>[2x]MGADDVVDSSKSFVMENFSSYHGTKPGYVDSIQKGIQKPKSGTQGNYDDDWEGFYSTDNKYDAAGYSVDNENPLSGKAGGVVKVTYPGLTKVLALKVDNAETIKKELGLSLTEPLMEQVGTEEFIKRFGDGASRVVLSLPFAEGSSSVKYINNWEQAKALSVELEINFETRGKRGQDAMYEYMAQACAGNRVRRSVGSSLSCINLDWDVIRDKTKTKIESLKEQGPIKNKMSESPNKTVSEEKAKQYLEEFHQTALEQPELSELKTVTGTNPVFAGANYAAWAVNVAQVIDSETADNLEKTTAALSILPGIGSVMGIADGAVHHNTEEIVAQSIALS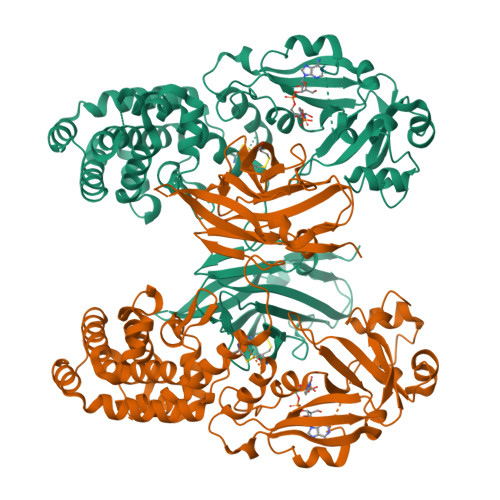SLMVAQAIPLVGELVDIGFAAYNFVESIINLFQVVHNSYNRPAYSPGHKTQPFLHDGYAVSWNTVEDSIIRTGFQGESGHDIKITAENTPLPIAGVLLPTIPGKLDVNKSKTHISVNGRKIRMRCRAIDGDVTFCRPKSPVYVGNGVHANLHVAFHRSSSEKIHSNEISSDSIGVLGYQKTVDHTKVNSKLSLFFEIKSMA>[4x]SNAMVMAPLPPVESLSLRQAIAQMIVVRGAGYLFDYERPYPQWEADQTTLQRWIEAGIGGVILLGGSAAEVAQKTKQLQSWAEIPLLIAADIEEGVGQRFRGATEFPPPMAFGEIWRTDPHQAIALAETMGATTAQEALSLGINWVLAPVLDVNNNPHNPVINIRAFGETPDQVSALGTAFIRGAQQYAVLTTAKHFPGHGDTATDSHLALPTISHD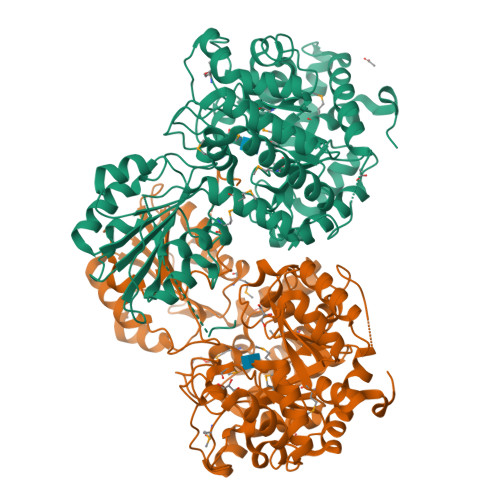DTRLNTVELPPFKAAIQGGVDAVMNAHLMIPAWDQQYPATLSPAILTGQLRHKLGFKGLIVTDALVMGGITQFAAPDTVVVQAIAAGADILLMPPDVDGAIIAIETAIKTGQLSESRIYESVERIWQAKQKILTATPSTFPQGISGDRPETRKTVAMVLERATKHQKSLVKISSFPDNFARNLIVVDSVLKSPFLRPNCPAIAIPQRHGYAAEIVELKTLPRLQLEAIPTLIQCFLRGNPFTEKLADPIDVLQKIAAQIPLQGVIFYGSPYFLEALQTTLPEIPWWFSYGQMAIAQAEICTSLWEEAPQAAPSAAEFI>[2x]MKKVRLKELESRLQQVDGFEKPKLLLEQYPTRPHIAACMLYTIHNTYDDIENKVVADLGCGCGVLSIGTAMLGAGLCVGFDIDEDALEIFNRNAEEFELTNIDMVQ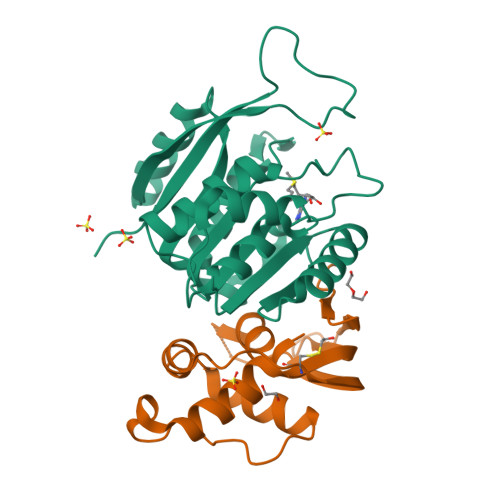CDVCLLSNRMSKSFDTVIMNPPFGTKNNKGTDMAFLKTALEMARTAVYSLHKSSTREHVQKKAAEWKIKIDIIAELRYDLPASYKFHKKKSVDIEVDLIRFSFHHHHHH;>[2x]MKLLTHNLLSSHVRGVGSRGFPLRLQATEVRICPVEFNPNFVARMIPKVEWSAFLEAADNLRLIQVPKGPVEGYEENEEFLRTMHHLLLEVEVIEGTLQCPESGRMFPISRGIPNMLLSEEETES>MDAWLQQTVFRGTLSISQGVDDRDLLLAPKWISFLSLSSFLKQKLLSLLRQIRELRLTTTVYPPQDKLMWWSHCCDPEDIKVVILGQDPYHKGQATGLAFSVDPQCQVPPSLRSIFRELEASVPNFSTPSHGCLDSWARQGVLLLNTVLTVEKGRAGSHEGLGWDWFTSFIISSISSKLEHCVFLLWGRKAIDRTPLINAQKHLVLTAQHPSPLASLGGRHSRWPRFQGCNHFNLANDYLTRHRRETVDWGLLEQ[8x];>[8x]MTL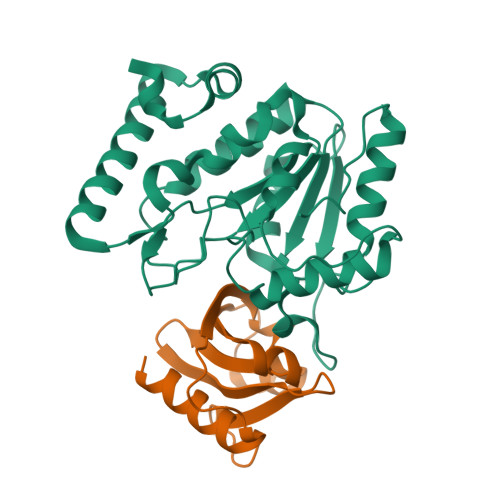ELQLKHYITNLFNLPKDEKWECESIEEIADDILPDQYVRLGALSNKILQTYTYYSDTLHESNIYPFILYYQKQLIAIGYIDENHDMDFLYLHNTIMPLLDQRYLLTGGQ>MDWVVAPISVPENGKGPFPQRLNQLKSNKDRDTKIFYSITGPGADSPPEGVFAVEKETGWLLLNKPLDREEIAKYELFGHAVSENGASVEDPMNISIIVTDQNDHKPKFTQDTFRGSVLEGVLPGTSVMQVTATDEDDAIYTYNGVVAYSIHSQEPKDPHDLMFTIHRSTGTISVISSGLDREKVPEYTLTIQAT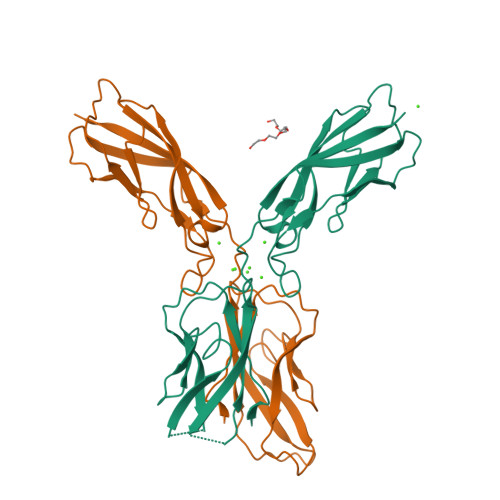DMDGDGSTTTAVAVVEILD[2x]> MHHHHHHMTTTQTAKASRRARIERRTRESDIVIELDLDGTGQVAVDTGVPFYDHMLTALGSHASFDLTVRATGDVEIEAHHTIEDTAIALGTALGQALGDKRGIRRFGDAFIPMDETLAHAAVDLSGRPYCVHTGEPDHLQHTTIAGSSVPYHTVINRHVFESLAANARIALHVRVLYGRDPHHITEAQYKAVARALRQAVEPDPRVSGVPSTK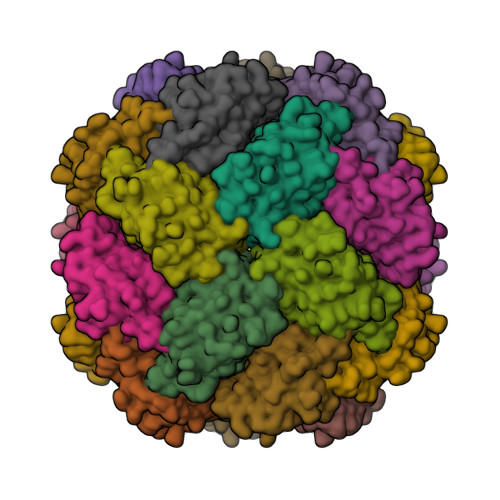GAL>MKIEEVKSTTKTQRIASHSHVKGLGLDESGLAKQAASGLVGQENAREACGVIVELIKSKKMAGRAVLLAGPPGTGKTALALAIAQELGSKVPFCPMVGSEVYSTEIKKTEVLMENFRRAIGLRIKETKEVYEGEVTELTPCETENPMGGYGKTISHVIIGLKTAKGTKQLKLDPSIFESLQKERVEAGDVIYIEANSGAVKRQGRCDTYATEFDLEAEEYVPLPKGDVHKKKEIIQDVTLHDLDVANARPQGGQDILSMMGQLMKPKKTEITDKLRGEINKVVNKYIDQGIAELVPGVLFVDEVHMLDIECFTYLHRALESSIAPIVIFASNRGNCVIRGTEDITSPHGIPLDLLDRVMIIRTMLYTPQEMKQIIKIRAQTEGINISEEALNHLGEIGTKTTLRYSVQLLTPANLLAKINGKDSIEKEHVEEISELFYDAKSSAKILADQQ[6x];>[6x]MATVTATTKVPEIRDVTRIERIGAHSHIRGLGLDDALEPRQASQGMVGQLAARRAAGVVLEMIREGKIAGRAVLIAGQPGTGKTAIAMGMAQALGPDTPFTAIAGSEIFSLEMSKTEALTQAFRRSIGVRIKEETEIIEGEVVEIQIDRPATGTGSKVGKLTLKTTEMETIYDLGTKMIESLTKDKVQ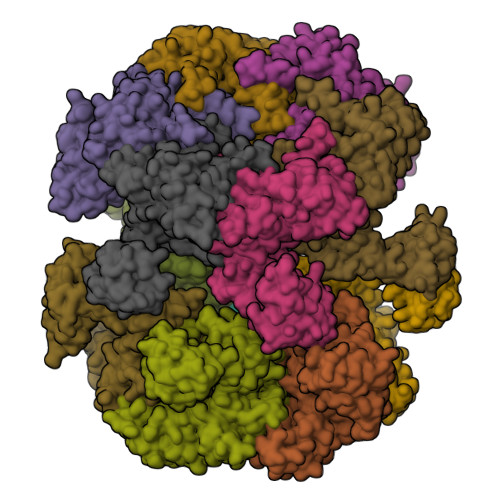AGDVITIDKATGKISKLGRSFTRARDYDAMGSQTKFVQCPDGELQKRKEVVHTVSLHEIDVINSRTQGFLALFSGDTGEIKSEVREQINAKVAEWREEGKAEIIPGVLFIDEVHMLDIESFSFLNRALESDMAPVLIMATNRGITRIRGTSYQSPHGIPIDLLDRLLIVSTTPYSEKDTKQILRIRCEEEDVEMSEDAYTVLTRIGLETSLRYAIQLITAASLVCRKRKGTEVQVDDIKRVYSLFLDESRSTQYMKEYQDAFLFNELKGETMDTS> ADPRLGQFELEILSMQNVNGELQNGNCCGGARNPGDRKCTGDECNTYFKVCLKEYQSRVRAGGPCSFGSGSTPVIGGNTFNLKASRGNDRNRIVLPFSFAWPRSYTLLVEAWDSSNDTIQPDSIIEKASHSGMINPSRQWQTLKQNTGIAHFEYRIRVTCDDHYYGFGCNKFC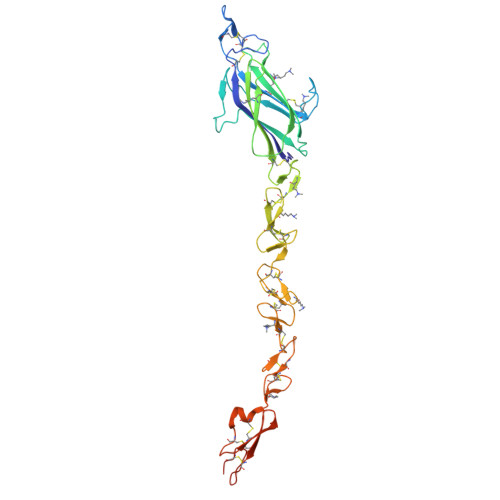RPRDDFFGHYACDQNGNKTCMEGWMGPECNKAICRQGCSPKHGSCKLPGDCRCQYGWQGLYCDKCIPHPGCVHGTCNEPWQCLCETNWGGQLCDKDLNYCGTHQPCLNRGTCSNTGPDKYQCSCPEGYSGPNCEAAAHHHHHHHH>SGMEKALEAARKAIEEHPEEAKEVAELNKKAGEIVKEAGSYEEVAKKVLELAREGKLSDDAIIAAAKGLAYDEEGQEVALKTAEEARKAAEESSGKGKERLTLLSFLLRLQVRLTRESEDDEGYLTLATVYWLAAKIAKKKLEEDPSASTDLEGIEKAFEEGLEEAKKAPEEEILKAGFDYFEKAKEIMEKGNKELRELLFK[2x]

Here we present rotamer inverted fragment finder–diffusion (Riff-Diff), a hybrid machine learning and atomistic modelling strategy for scaffolding catalytic arrays in de novo proteins. We highlight the general applicability of Riff-Diff by designing enzymes for two mechanistically distinct chemical transformations, the retro-aldol reaction and the Morita–Baylis–Hillman reaction. We show that in both cases, it is possible to generate catalysts that exhibit activities rivalling those optimized by in vitro evolution, along with exquisite stereoselectivity. High-resolution structures of six of the designs revealed near-atomic active site design precision.

We obtained crystal structures of the four designs: RAD13 (kcat = 3.8 × 10−5 s−1), RAD17 (kcat not determined), RAD32 (kcat = 1.1 × 10−2 s−1), and RAD36 (kcat = 6.2 × 10−5 s−1). The crystal structures agree with the design models, having backbone Cα RMSD values between 0.68 Å and 1.2 Å. The catalytic residues of RAD13 and RAD17 adopted the correct conformation with heavy-atom sidechain RMSD values of 0.42 Å and 1.09 Å to the design model and 0.89 Å and 1.2 Å to the catalytic geometry, respectively. Despite the near-atomic precision with which the tetrad was reproduced, RAD13 and RAD17 were more than 105-fold slower than RA95.5-8F. This indicates that precise positioning of catalytic sidechains is by itself not sufficient to design efficient biocatalysts, even when scaffolding catalytic arrays that are derived from highly active enzymes. RMSD is a popular metric for measuring how closely a designed active site aligns with the intended catalytic array, but it is agnostic to the geometric constraints of catalytic interactions. This could explain the discrepancy between the low RMSD in the active site of RAD13 and low catalytic activity and general poor predictiveness of sidechain RMSD for activity.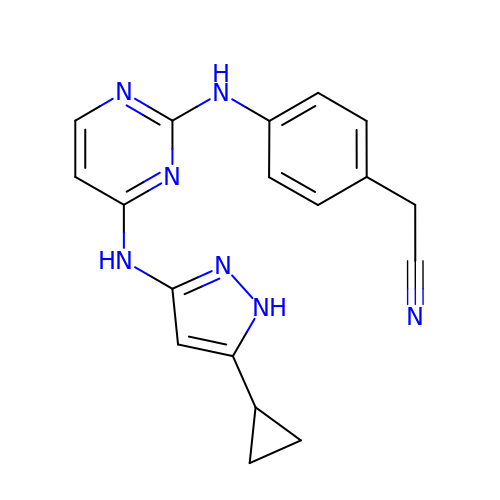[4-({4-[(5-cyclopropyl-1H-pyrazol-3-yl)amino]pyrimidin-2-yl}amino)phenyl]acetonitrile | C18 H17 N7 | YRRRHSNOXWKVDL-UHFFFAOYSA-N> HMRKIIVGSRRSKLALTQTKWVIEQLKKQGLPFEFEIKEMVTKGDQILNVTLSKVGGKGLFVKEIEQAMLDKEIDMAVHSMKAMPAVLPEGLTIGCIPL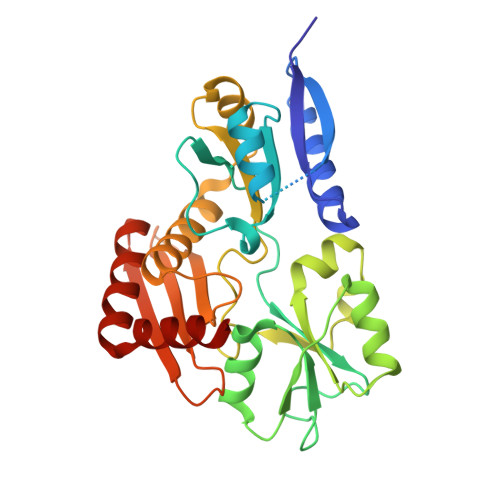REDHRDALISKNGERFEELPSGAVIGTSSLRRGAQLLSMRSDIEIKWIRGNIDTRLEKLKNEDYDAIILAAAGLSRMGWSKDTVTQYLEPEISVPAVGQGALAIECRENDHELLSLLQALNHDETARAVRAERVFLKEMEGGCQVPIAGYGRILDGGNIELTSLVASPDGKTIYKEHITGKDPIAIGSEAAERLTSQGAKLLIDRVKEELDK>[4x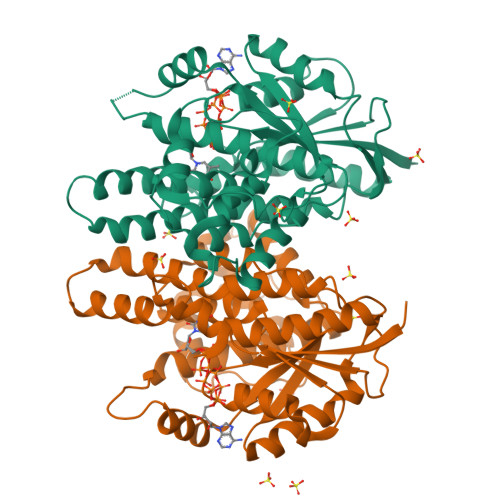]GSHMVTIVRIYLDGVYGIGKSTTGRVMASAASGGSPTLYFPEPMAYWRTLFETDVISGIYDTQNRKQQGNLAVDDAALITAHYQSRFTTPYLILHDHTCTLFGGNSLQRGTQPDLTLVFDRHPVASTVCFPAARYLLGDMSMCALMAMVATLPREPQGGNIVVTTLNVEEHIRRLRTRARIGEQIDITLIATLRNVYFMLVNTCHFLRSGRVWRDGWGELPTSCGAYKHRATQMDAFQERVSPELGDTLFALFKTQELLDDRGVILEVHAWALDALMLKLRNLNVFSADLSGTPRQCAAVVESLLPLMSSTLSDFDSASALERAARTFNAEMGV In summary, our study demonstrates that PH0208 protein would function as a purine nucleotide dependent R15Pi enzyme and not as a homologue of the regulatory subunit of eIF2B. In NMP degradation pathway, R15Pi catalyzes the conversion of ribose-1,5-bisphosphate (R15P, substrate) into ribulose-1,5-bisphosphate (RuBP, product) in an adenosine 5′-monophosphate (AMP)-dependent manner. AMP acts as an activator of R15Pi and in its absence the enzymatic activity has been found to decline dramatically. Monomer of PH0208 protein consists of an N-terminal α-helical domain (residues 1–122) and a C-terminal α-β-α sandwich domain (residues 123–324).

The other catalytic residue, Asp204, reported to be vital for ligand binding in R15Pi enzyme was mutated to asparagine. However, quite surprisingly, a clear electron density of the substrate was still observed at the active site pocket of the PH0208-D204N mutant protein. The interactions involved in holding R15P in the active site pocket of PH0208-D204N mutant protein are equivalent to those of the PH0208-WT and PH0208-C135S proteins. The absence of electron density of R15P in the active site pocket of D202N (D204 in PH0208) mutant of R15Pi from T. kodakarensis led to the proposition that this residue might play an essential role in ligand binding. Interestingly, the PH0208-D204N mutant held the substrate at the active site pocket indicating that the residue aspartate alone is not responsible for ligand binding and there might be other criteria that govern the binding of the ligand. Therefore, binding affinity was studied using the mutant proteins, PH0208-C135S and PH0208-D204N in which case the heat change would be solely due to ligand binding. The analysis shows that both PH0208-C135S and PH0208-D204N proteins bind to R15P with high affinity with equilibrium dissociation constants (Kd) of 13.8 and 10 μM, respectively. On the contrary, the PH0208-C135S and PH0208-D204N bind the product (RuBP) with negative ∆H value for the binding peaks indicating an exothermic reaction. The mutants formed strong interactions with RuBP with Kd values of 7.5 and 7.2 μM, respectively, which corresponds to the binding affinity of the substrate.

>[3x]MGAMIVKEVYETAEKIKSMEIRGAGRIARAAAQALMIQAEKSKAKEPEELWNELKVASKILYNTRPTAVSLPNALRYVMHRVKAAYLGGADLETLRFTAINSAKEFIYNSEKAIERIGEIGAKRIEDGDIIMTHCHSKAAISVMKKAFEQGKNIKVIVTETRPKWQGKITAKELASYGIPVIYIVDSAARHYMKMTDKVVMGANSITANGAVINKIGTSLIALTAKEHRVWVMIAAETYKFHPATMLGQLVEIEMRDPTEVIPEEELRTWPKNIEVWNPAFDVTPPEYIDVIITERGIIPPYAAIDILKEEFGWALKYKEPWED> HMKELKYDVLIIGGGFAGSSAAYQLSRRGLKILLVDSKPWNRIGDKPCGDAVSKAHFDKLGMPYPKGEELENKINGIKLYSPDMQTVWTVNGEGFELNAPLYNQRVLKEAQDRGVEIWDLTTAMKPIFEDGYVKGAVLFNRRTNEELTVYSKVVVEATGYSRSFRSKLPPELPITEDLDDKDADVAYREVLLTKEDIEDHDYLRIFFDQETSPGGYWWYFPKGKNKVNVGLGIQGGMGYPSIHEYYKKYLDKYAPDVDKSKLLVKGGALVPTRRPLYTMAWNGIIVIGDSGFTVNPVHGGGKGSAMISGYCAAKAILSAFETGDFSASGLWDMNICYVNEYGAKQASLDIFRRFLQKLSNDDINYGMKKKIIKEEDLLEASEKGDLHLSVADKAMRVISGLGRPSLLFKLKAVAESMKKIKELYLNYPRSPSSLGSWRR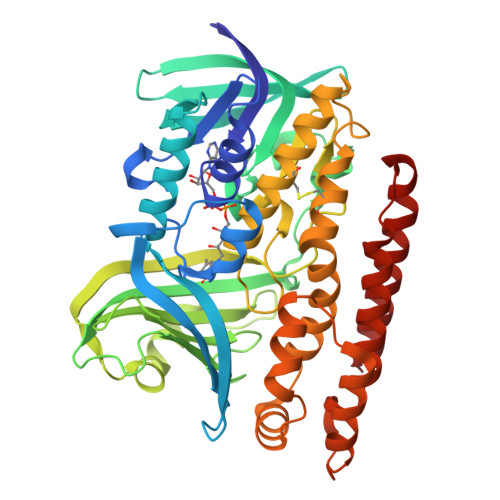EVDNVLTEFNKSLS> MKVLEERNAFLSDYEVLKFLTDLEKKHLWDQKSLAALKKSRS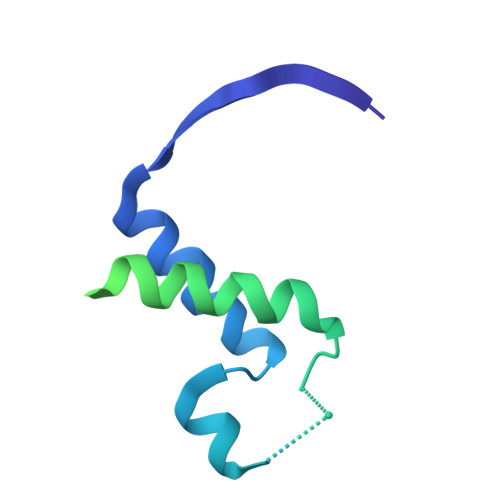KGKQNRPYNHPELQGITRNVVNYLSINKNFINQEDEGEERESSGAKDAEKSGISKMSDESFAELMTKLNSFKLFKAEKLQIVNQLPANMVHLYSIVEECDARFDEKTIEEMLEIISAYA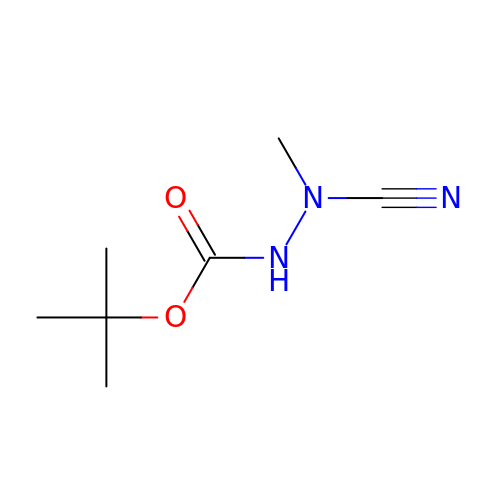TERT-BUTYL 2-CYANO-2-METHYLHYDRAZINECARBOXYLATE | C7 H13 N3 O2 | SWELYBAPJHIOQT-UHFFFAOYSA-N>SNASRDDKKDGVAGPGDAVRVTSSKLVTQPGTSNPKAVVSFYEDFLCPACGIFERGFGPTVSKLVDIGAVAADYTMVAILDSASNQHYSSRAAAAAYCVADESIEAFRRFHAALFSKDIQPAELGKDFPDNARLIELAREAGVVGKVPDCINSGKYIEKVDGLAAAVNVHATPTVRVNGTEYEWSTPAALVAKIKEIVGDVPGIDSAAATATS[2x]

Here, the Mtb protein Rv2969c is investigated and it is shown that it is the DsbA-like partner protein of MtbVKOR. It is found that it has the characteristic redox features of a DsbA-like protein: a highly acidic catalytic cysteine, a highly oxidizing potential and a destabilizing active-site disulfide bond. Rv2969c also has peptide-oxidizing activity and recognizes peptide segments derived from the periplasmic loops of MtbVKOR. The crystal structure of Rv2969c reveals a canonical DsbA fold comprising a thioredoxin domain with an embedded helical domain.

To explore the atomic details of MtbDsbA, we determined its structure at 2.0 Å resolution. The two MtbDsbA molecules in the asymmetric unit are very similar (r.m.s. deviation of 0.26 Å for all Cα atoms). As in all thioredoxin-like proteins, the catalytic CXXC motif is located at the N-­terminus of helix H1 in MtbDsbA. However, the catalytic motif (Cys89-Pro90-Ala91-Cys92) in MtbDsbA differs from other structurally characterized DsbAs, which are generally Cys-Pro-His/Tyr/Ser-Cys. The active-site disulfides of DsbA proteins are susceptible to radiation damage in the crystal and the broken disulfide bond in MtbDsbA is therefore likely to be a result of the synchrotron radiation used to measure the diffraction data. Ordered active-site water molecules are present in the crystal structure at positions consistent with formation of stabilizing hydrogen bonds to the Cys89 thiolate and to Thr214, a residue preceding the cis-Pro loop. Helix H8 at the C-terminus of MtbDsbA and its interaction with active-site helix H1 are unique to MtbDsbA among structurally characterized DsbAs. Compared with other structurally characterized DsbAs, the presence of helix H8 in MtbDsbA buries a greater proportion of helix H1 (buried surface area of 592 versus 401–260 Å2). The H8 helix interaction may restrict the conformational flexibility of helices H1 and H7. Unexpectedly, a ligand, 1,4-dioxane from the crystallization solution, was bound in this shallow groove, forming contacts with Ile94, Gly98, Phe99 and Pro229.> AGVMTGAKFTQIQFGMTRQQVLDIAGAENCETGGSFGDSIHCRGHAAGDYYAYATFGFTSAAADAKVDSKSQEKLLAPSAPTLTLAKFNQVT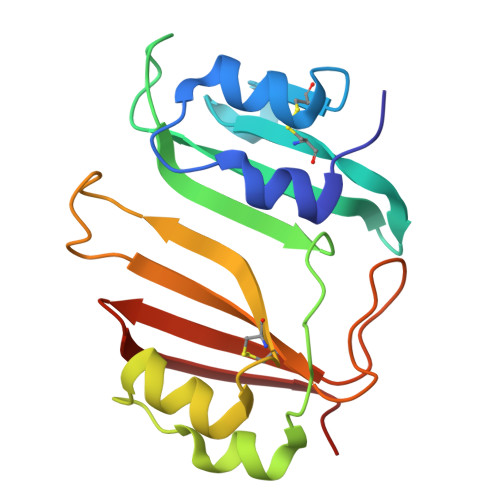VGMTRAQVLATVGQGSCTTWSEYYPAYPSTAGVTLSLSCFDVDGYSSTGFYRGSAHLAFTDGVLQGKRQWDLV>SNASRSYNDELQFLEKINKNCWRIKKGFVPNMQVEGVFYVNDALEKLMFEELRNACRGGGVGGFLPAMKQIGNVAALPGIVHRSIGLPDVHSGYGFAIGNMAAFDMNDPEAVVSPGGVGFDINCGVRLLRTNLDESDVQPVKEQLAQAMFDHIPVGVGSKGVIPMNAKDLEEALEMGVDWSLREGYAWAEDKEHCEEYGRMLQADPNKVSARAKKRGLPQLGTLGAGNHYAEIQVVDEIFNEYAAKKMGIDHKGQVCVMIHSGSRGLGHQVATDALVAMEKAMKRD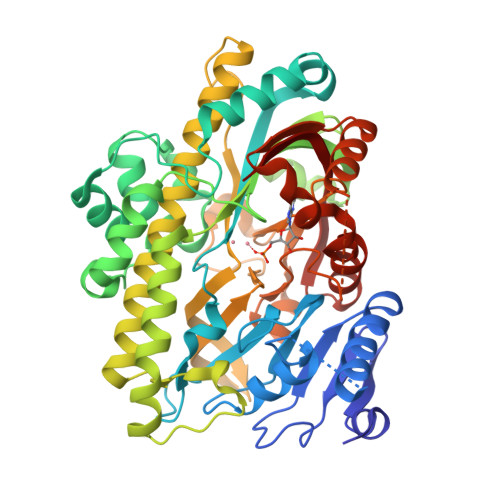KIIVNDRQLACARIASPEGQDYLKGMAAAGNYAWVNRSSMTFLTRQAFAKVFNTTPDDLDLHVIYDVSHNIAKVEQHVVDGKERTLLVHRKGSTRAFPPHHPLIAVDYQLTGQPVLIGGTMGTCSYVLTGTEQGMTETFGTTCHGAGRALSRAKSRRNLDFQDVLDKLADMGIAIRVASPKLVMEEAPESYKNVTDVVNTCHDAGISKKAIKLRPIAVIKG[2x]> SNRDLFAELSSALVEAKQHSEGKLTLKTHHVNDVGELNISPDEIVSIREQFNMSRGVFAR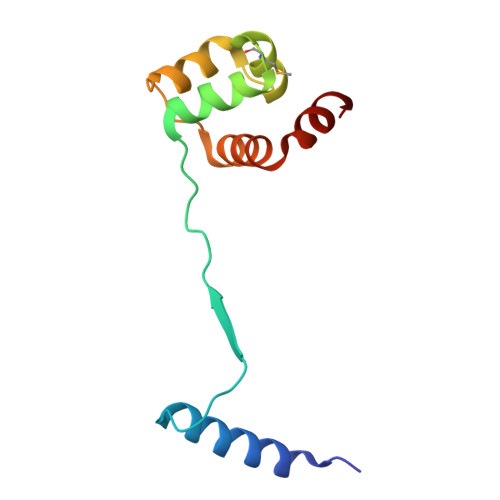LLHTSSRTLENWEQGRSVPNGQAVTLLKLVQRHPETLSHIAEL> MAYVEIIEQPKQRGMRFRYKCEGRS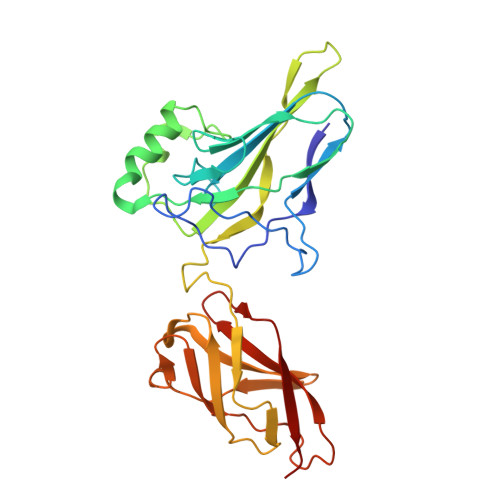AGSIPGERSTDTTKTHPTIKINGYTGPGTVRISLVTKDPPHRPHPHELVGKDCRDGYYEADLCPDRSIHSFQNLGIQCVKKRDLEQAISQRIQTNNNPFHVPIEEQRGDYDLNAVRLCFQVTVRDPAGRPLLLTPVLSHPIFDNRAPNTAELKICRVNRNSGSCLGGDEIFLLCDKVQKEDIEVYFTGPGWEARGSFSQADVHRQVAIVFRTPPYADPSLQAPVRVSMQLRRPSDRELSEPMEFQYLPD GAMMA-GLUTAMYL[S-(2-IODOBENZYL)CYSTEINYL]GLYCINE 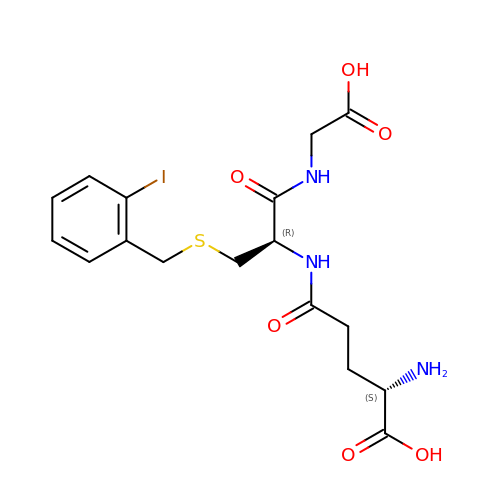| C17 H22 I N3 O6 S | QFYJAEOZTBVJQM-STQMWFEESA-N>ARGDGRRRG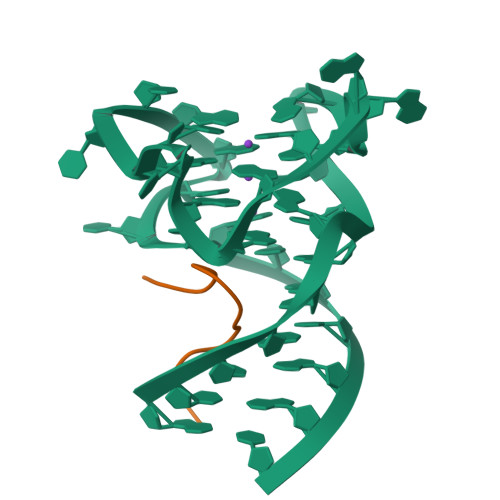GGGRGQGGR[2x]>[3x]SGLVESGTLWDHYTLNILEANETQRGTLRVATQVEAAAGTLDNVLITPKKLLGTKSTEAQEGVIKVATQSETVTGTSANTAVSPKNLKWIAQSEPTWAATTAIRGFVKTSSGSITFVGNDTVGSTQDLELYEKNSYAVSPYELNRVLANYLPLKAKAADTNLLDGLDSSQFIRRDIAQTVNGSLTLTQQTNLSAPLVSSSTGEFGGSLAANRTFTIRNTGAPTSIVFEKGPASGANPAQSMSIRVWGNQFGGGSDTTRSTVFEVGDDTSHHFYSQRNKDGNIAFNINGTVMPININASGLMNVNGTATFGRSVTANGEFISKSANAFRAINGDYGFFIRNDASNTYFLLTAAGDQTGGFNGLRPLLINNQSGQITIGEGLIIAKGVTINSGGLTVNSRIRSQGTKTSDLYTRAPTSDTVGFWSIDINDSATYNQFPGYFKMVEKTNEVTGLPYLERGEEVKSPGTLTQFGNTLDSLYQDWITYPTTPEARTTRWTRTWQKTKNSWSSFVQVFDGGNPPQPSDIGALPSDNATMGNLTIRDFLRIGNVRIVPDPVNKTVKFEWVE

The proximal half-fiber is formed by a parallel homo-trimer of gp34. The protein is a highly intertwined trimer containing a 2 nm-wide triple β-helix domain interspersed with three wider domains in which each of the monomers forms an anti-parallel β-sheet. The long tail fibers recognize the outer membrane protein C (OmpC) or the lipopolysaccharide (LPS) of E. coli and are responsible for the initial and reversible attachment of the virion. The carboxy-terminal parts of gp34 that we crystallized occupy the part of the proximal tail fiber closest to gp35 (the “knee”).

The structures of gp34(781–1289) and gp34(726–1289) were also solved by molecular replacement, both with one trimer in the asymmetric unit and belonging to the P21 space group. The gp34(726–1289) structure was composed of 1668 residues (744–1289 in each of the three chains), a glycerol, and 350 water molecules. The N-termini of gp34(726–1289) and gp34(781–1289) are less well ordered in the crystal structures, presumably due to flexibility and lack of crystal contacts in these regions. The structure of the carboxy-terminal part of gp34 reveals an elongated protein; just over 30 nm long for the longest crystallographic model, containing residues 744–1289. The longest structure, gp34(744–1289), was fitted into the reconstructed electron microscopy (EM) map of the extended T4 tail. Although the density for the long tail fiber is not as clear as for the other parts of the tail, it was possible to fit the crystal structure manually into the density by using domains P3, P4, and P5 as an indicator. The crystal structure is slightly bent around residue 881. The EM density for the gp34 fiber is also curved. Thus, we think the bending is a feature of this protein. Gp34 residues 744–776, 780–812, 823–868, and gp12 182–215 can be superimposed nicely, and the repeating sequences are well-conserved.> MISLNGYGRFG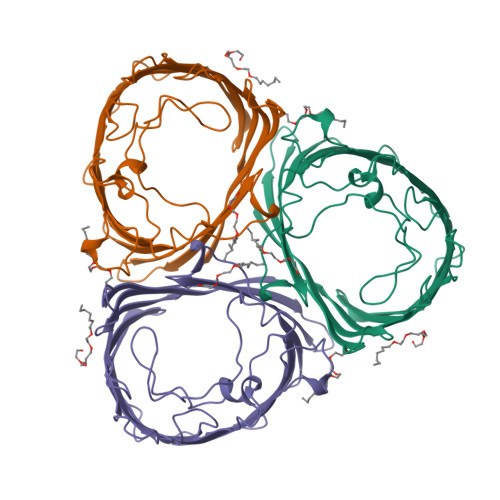LQYVEDRGVGLEDTIISSRLRINIVGTTETDQGVTFGAKLRMQWDDGDAFAGTAGNAAQFWTSYNGVTVSVGNVDTAFDSVALTYDSEMGYEASSFGDAQSSFFKYNSKYDASGALDNYNGIAVTYSISGVNLYLSYVDPDQTVDSSLVTEEFGIAADWSNDMISLAAAYTTDAGGIVDNDIAFVGAAYKFNDAGTVGLNWYDNGLSTAGDQVTLYGNYAFGATTVRAYVSDIDRAGADTAYGIGADYQFAEGVKVSGSVQSGFANETVADVGVRFDF>SDFANLSSTNKELSPQYNWVACGILEGGLKAAGVLEEGQYNRELAEAIAAKGEGFWTTQFPQIGDWNEDQAAALADRAQ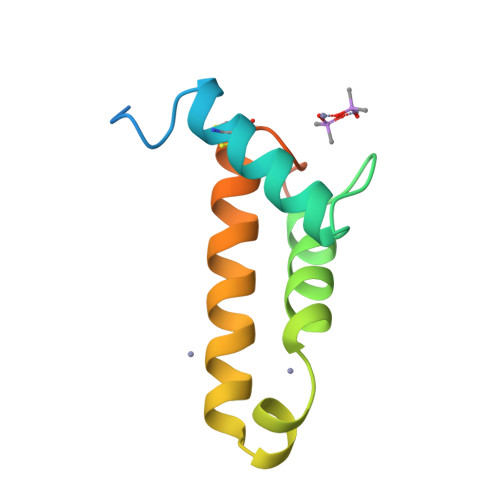TCGLVKADTYLSELSSNFSS[2x]(2~{S})-2-(3-azanylpropanoylamino)-3-(3-methylimidazol-4-yl)propanoic acid | C10 H16 N4 O3 | 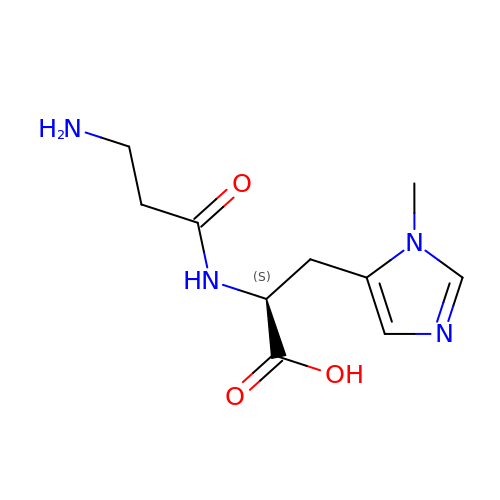MYYIAHXIVFADCU-QMMMGPOBSA-N> QEKRKQISVRGLAGVENVTELKKNFNRHLHFTLVKDRNVATPRDYYFALAHTVRDHLVGRWIRTQQHYYEKDPKRIYYLSLEFYMGRTLQNTMVNLALENACDEATYQLGLDMEELEEIEEDAGLGNGGLGRLAACFLDSMATLGLAAYGYGIRYEFGIFNQKICGGWQMEEADDWLRYGNPWEKARPEFTLPVHFYGRVEHTSQGAKWVDTQVVLAMPYDTPVPGYRNNVVNTMRLWSAKAPNDFNLKDFNVGGYIQAVLDRNLAENISRVLYPNDNFFEGKELRLKQEYFVVAATLQDIIRRFKSSKFGCRDPVRTNFDAFPDKVAIQLNDTHPSLAIPELMRVLVDLERLDWDKAWEVTVKTCAYTNHTVIPEALERWPVHLLETLLPRHLQIIYEINQRFLNRVAAAFPGDVDRLRRMSLVEEGAVKRINMAHLCIAGSHAVNGVARIHSEILKKTIFKDFYELEPHKFQNKTNGITPRRWLVLCNPGLAEIIAERIGEEYISDLDQLRKLLSYVDDEAFIRDVAKVKQENKLKFAAYLEREYKVHINPNSLFDVQVKRIHEYKRQLLNCLHVITLYNRIKKEPNKFVVPRTVMIGGKAAPGYHMAKMIIKLITAIGDVVNHDPVVGDRLRVIFLENYRVSLAEKVIPAADLSEQISTAGTEASGTGNMKFMLNGALTIGTMDGANVEMAEEAGEENFFIFGMRVEDVDRLDQRGYNAQEYYDRIPELRQIIEQLSSGFFSPKQPDLFKDIVNMLMHHDRFKVFADYEEYVKCQERVSALYKNPREWTRMVIRNIATSGKFSSDRTIAQYAREIWGVEPSRQRLPA

Glycogen phosphorylase (GP; EC 2.4.1.1) is the enzyme that catalyzes the first step of glycogenolysis toward the production of glucose-1-phosphate. GP is an allosteric enzyme according to the Wyman–Monod–Changeux model and, through effector binding, adopts two interconverting states, a low-activity (T) state and a high-activity (R) state. GP has several ligand-binding sites that can be exploited for inhibitor binding. The structures of rmGPb-EGCG and rmGPb-EGC complexes were determined by X-ray crystallography, showing binding at the quercetin binding site (QBS) in agreement with kinetic studies that revealed both compounds as noncompetitive inhibitors of GP, with EGCG also causing a significant reduction in cell viability and migration of U87-MG glioblastoma cells.

Κinetic experiments with rmGPb and rmGPa showed that EGCG potently inhibited GP Ki = 49.8 ± 1.6 μM for rmGPb and Ki = 46.7 ± 1.4 μΜ for rmGPa, hence having similar affinity for both muscle GP forms. The QBS is located close to the protein surface about 15 Å from the active site, 43 Å from the allosteric site, and 32 Å from the inhibitor site. It forms a groove constellated by residues Lys544, Arg551, Lys655, and Tyr548 on one side and by Glu120 and Glu123 on the other side. Upon binding, EGCG makes a total of 107 van der Waals (vdw) interactions (14 polar–polar, 39 nonpolar–nonpolar, and 54 polar–non polar interactions). In addition, 2 water-mediated bridges with protein residues are formed, namely, O02-Wat1037-Cys495 (O) and O03-Wat1134-Asn541 (OD1). Aromatic rings A and B are positioned in 4.06 and 3.20 Å of positively charged Lys544 and Arg551, respectively, forming cation−π interactions. The gallate group (ring D) of EGCG forms 2 extra hydrogen bonds through its hydroxyl oxygens (O37) and (O44) compared with the nongallated EGC, with residues Tyr548 (N) and Glu120 (OE2), respectively. Superposition of the binary complexes of rmGPb-EGCG with rmGPb-EGC reveals a shift (RMSD, 3.31 Å) of the Glu120(OE2) side chain upon EGCG binding due to its hydrogen-bonding interaction with hydroxyl oxygen (O44) of the gallate group. In comparison to quercetin, EGCG having an extra ring (ring D) forms overall more vdw interactions (107 compared to 63 for quercetin).>MLFLIYRKDRPGSLQVRIDNYAAHLAYLEPLKAKIQVGGPTLGAGTGTDDKDMTGSFLIMEAESWDEVHSFVENDPFTKAGLFAATIVERWKH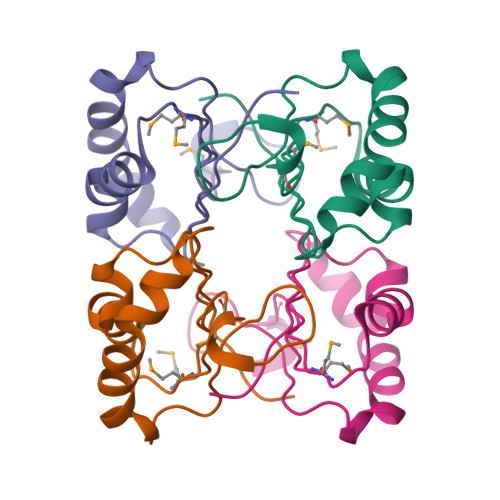GKHNDSK[4x]>PSYAVSSRAGLIDQERRAAVADLLTTLHRDIAVAPRYLVQVIFNDL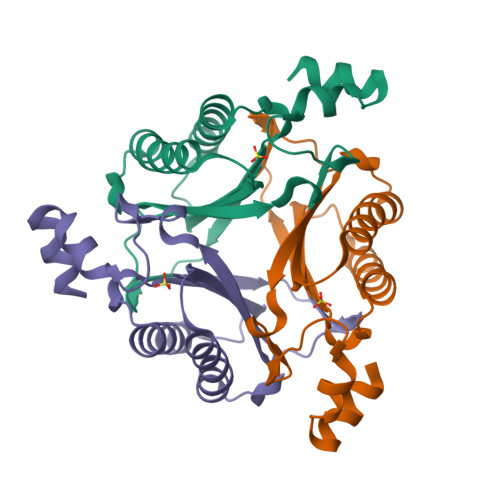DAGALFLAGREAPEGHVWIHADIRSGRTAQQKTDLLEQITSKVADVLELPPEHVWVYVNEIPGENMTEYGKLLPEPGKEEEWFATLPQSLQEELSDLR[3x]>[2x]MGFKQDIATLRGDLRTYAQDIFLAFLNKYPDEKRNFKNYVGK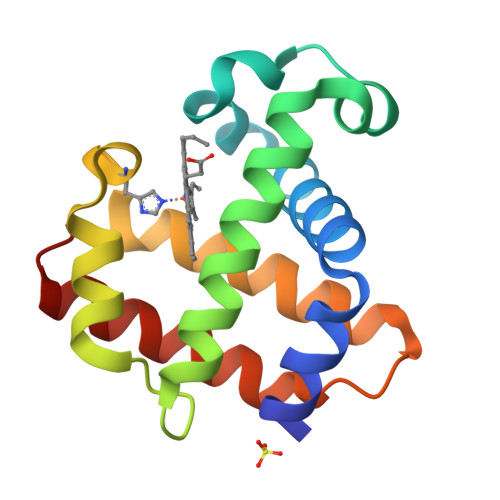SDQELKSMAKFGDHTEKVFNLMMEVADRATDCVPLASDASTLVQMKQHSGLTTGNFEKLFVALVEYMRASGQSFDSQSWDRFGKNLVSALSSAGMK> MDSTDLFDVFEETPVELPTDSNGEKNADTNVGDTPDHTQDKKHG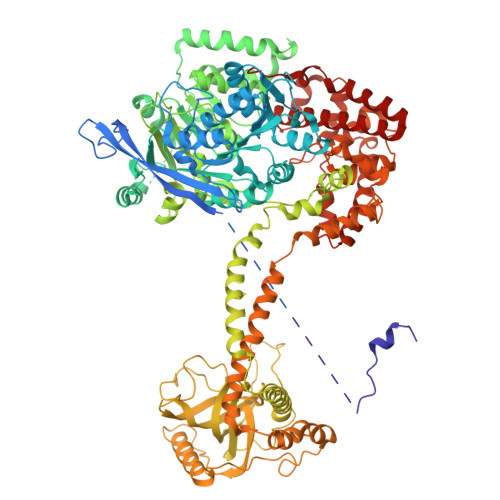LEEEKEEHEENNSENKKIKSNKSKTEDKNKKVVVPMLADSFEQEASREVDASKGLTNSETLQVEQDGKVRLSHQVRHQVALPPNYDYTPIAEHKRVNEARTYPFTLDPFQDTAISCIDRGESVLVSAHTSAGKTVVAEYAIAQSLKNKQRVIYTSPIKALSNQKYRELLAEFGDVGLMTGDITINPDAGCLVMTTEILRSMLYRGSEVMREVAWVIFDEVHYMRDKERGVVWEETIILLPDKVRYVFLSATIPNAMEFAEWICKIHSQPCHIVYTNFRPTPLQHYLFPAHGDGIYLVVDEKSTFREENFQKAMASISNQIGDDPNSTDSRGKKGQTYKGGSAKGDAKGDIYKIVKMIWKKKYNPVIVFSFSKRDCEELALKMSKLDFNSDDEKEALTKIFNNAIALLPETDRELPQIKHILPLLRRGIGIHHSGLLPILKEVIEILFQEGFLKVLFATETFSIGLNMPAKTVVFTSVRKWDGQQFRWVSGGEYIQMSGRAGRRGLDDRGIVIMMIDEKMEPQVAKGMVKGQADRLDSAFHLGYNMILNLMRVEGISPEFMLEHSFFQFQNVISVPVMEKKLAELKKDFDGIEVEDEENVKEYHEIEQAIKGYREDVRQVVTHPANALSFLQPGRLVEISVNGKDNYGWGAVVDFAKRINKRNPSAVYTDHESYIVNVVVNTMYIDSPVNLLKPFNPTLPEGIRPAEEGEKSICAVIPITLDSIKSIGNLRLYMPKDIRASGQKETVGKSLREVNRRFPDGIPVLDPVKNMKIEDEDFLKLMKKIDVLNTKLSSNPLTNSMRLEELYGKYSRKHDLHEDMKQLKRKISESQAVIQLDDLRRRKRVLRRLGFCTPNDIIELKGRVACEISSGDELLLTELIFNGNFNELKPEQAAALLSCFAFQERCKEAPRLKPELAEPLKAMREIAAKIAKIMKDSKIEVVEKDYVESFRHELMEVVYEWCRGATFTQICKMTDVYEGSLIRMFKRLEELVKELVDVANTIGNSSLKEKMEAVLKLIHRDIVSAGSLYL> MSRSGKSLTKYKIVFLGEQGVGKTSLITRFMYDTFDDHYQATIGIDFLSKTMYLDDKTIRLQLWDTAGQERFRSLIPSYIRDSRVAIIVYDITKRKSFEYIDKWIEDVKNERGDENVILCIVGNKSDLSDERQIST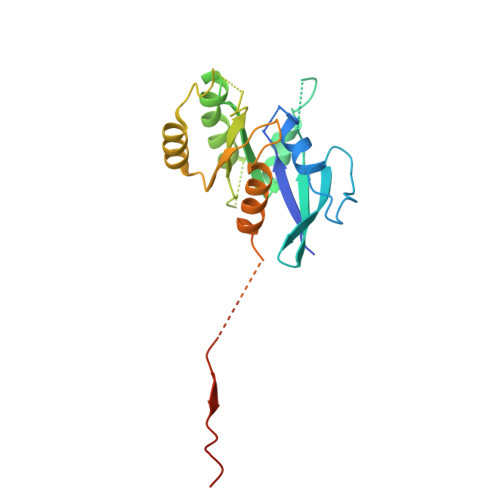EEGEKKAKLLGAKIFMETSTKAGYNVKALFKKIAKSLPEFQNSESTPLDSENANSANQNKPGVIDISTAEEQEQSACQC>[6x]MATLICGSIAYDNIMTFEGRFREHILPDQVHLINLSFLVPTMRREFGGCAGNIAYALNLLGGDARMMGTLGAVDAQPYLDRMDALGLSREYVRVLPDTYSAQAMITTDLDNNQITAFHPGAMMQSHVNHAGEAKDIKLAIVGPDGFQGMVQHTEELAQAG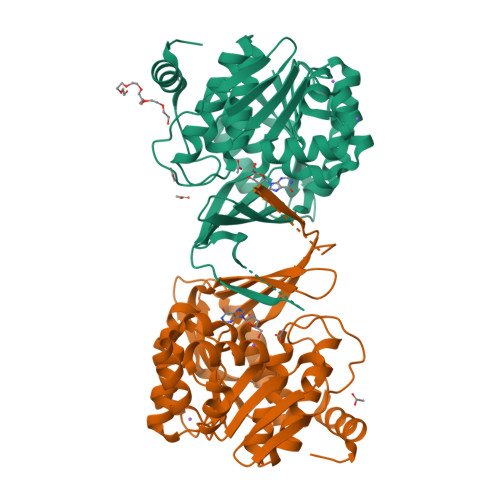VPFIFDPGQGLPLFDGATLRRSIELATYIAVNDYEAKLVCDKTGWSEDEIASRVQALIITRGEHGATIRHRDGTEQIPAVRAERVIDPTGCGDAFRGGLLYGIEHGFDWATAGRLASLMGALKIAHQGPQTYAPTRAEIDARFETAFGYRPKGSKLRSLEHHHHHH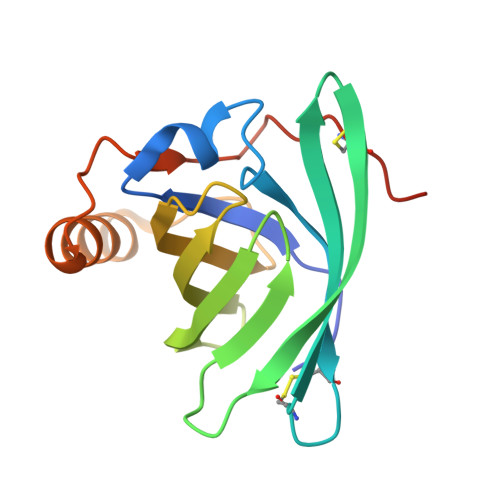>[5x]MAEINGDWNTIALSADNKEKIEEGGPLRVYFRQVDCNDDCSEITFRLYVKLSGECKESTVIASQTPDDFYTVQFAGENTFLIVDKQEDLFTLYNTNVDENGLVTRGYAIIGKRDSLTPEETSHFEEANELKGIPKGNIEYLAGTDDCPERSHHHHHH> LMTVSKFASICTMGANASALEKEIGPEQFPVNEHYFGLVNFGNTCYCNSVLQALYFCRPFREKVLAYKSQPRKKESLLTCLADLFHSIATQKKKVGVIPPKKFITRLRKENELFDNYMQQDAHEFLNYLLNTIADILQEERKQEKQNGRLPNGNIDNENNNSTPDPTWVHEIFQGTLTNETRCLTCETISSKDEDFLDLSVDVEQNTSITHCLRGFSNTETLCSEYKYYCEECRSKQEAHKRMKVKKLPMILALHLKRFKYMDQLHRYTKLSYRVVFPLELRLFNTSGDATNPDRMYDLVA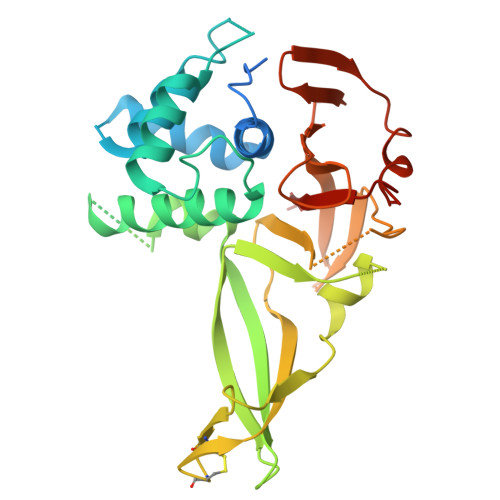VVVHCGSGPNRGHYIAIVKSHDFWLLFDDDIVEKIDAQAIEEFYGLTSDISKNSESGYILFYQSRD> MAWPKVQPEVNIGVVGHVDHGKTTLVQAITGIWTSKHSEELKRGMTIKLGYAETNIGVCESCKKPEAYVTEPSCKSCGSDDEPKFLRRISFIDAPGAEVLMATMLSGAALMDGAILVVAANEPFPQPQTREHFVALGIIGVKNLIIVQNKVDVVSKEEALSQYRQIKQFTKGTWAENVPIIPVSALHKINIDSLIEGIEEYIKTPYRDLSQKPVMLVIRSFDVNKPGTQFNELKGGVIGGSIIQGLFKVDQEIKVLPGLRVEKQGKVSYEPIFTKISSIRFGDEEFKEAKPGGLVAIGTYLDPSLTKADNLLGSIITLADAEVPVLWNIRIKYNLLERVVGAKEMLKVDPIRAKETLMLSVGSSTTLGIVTSVKKDEIEVELRRPVAVWSNNIRTVISRQIAGRWRMIGWGLVEI

In eukaryotic and archaeal cells, the initiator tRNA carrier is the e/aIF2 heterotrimer. In its GTP-bound form, this factor specifically binds Met-tRNAiMet and brings it to the initiation complex. The γ subunit forms the core of the heterotrimer and contains the GTP-binding pocket. α and β are bound to γ but do not interact together. We were able to observe GTP hydrolysis by aIF2 or by its isolated γ subunit.

H97A and D19A mutants were crystallized in the same conditions as those used for wt-aIF2γ but in the presence of GTP-Mg2+. In keeping with the observed decreased rates of GTP hydrolysis, we observed that GTP was intact within the crystals grown at 4°C. In the D19A-GTP4 and H97A-GTP4 structures, GTP is tightly bound to the canonical nucleotide-binding pocket in a position similar to that of GDPNP in wt-aIF2γ. Unexpectedly in H97A-GTP4 structure, a second magnesium ion (hereafter named Mg2) is observed within the nucleotide-binding pocket. The octahedral coordination of the second magnesium ion is clearly visible. Four water molecules form the equatorial plane. One of these water molecules also interacts with oxygen atoms of the α, β and γ phosphate groups of GTP. In apical positions are the side chain of D19 and the carbonyl group of G44. No alternate conformation of D19 is observed showing that the residue is now tightly stabilized. Accordingly, the high quality electron density maps suggested that in H97A-GTP4, a very small fraction of GTP was converted into GDP-Pi. Strikingly, the position of the catalytic arginine residue of RasGAP (R789) matches that of the second magnesium ion bound to D19.> 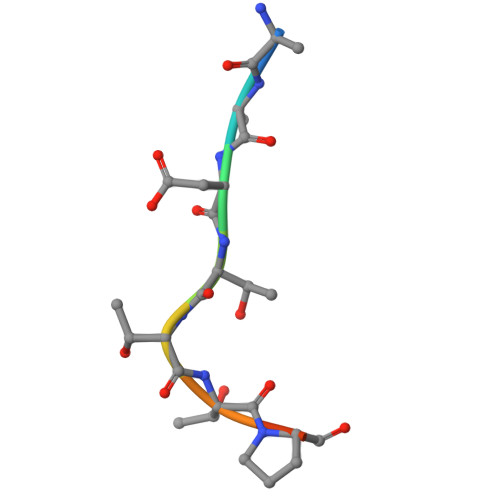KADTTTPTT> MCASRDDWRCARSMHEFSAKDIDGHMVNLDKYRG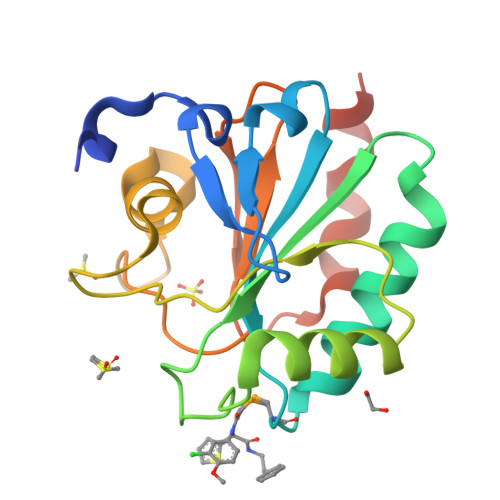FVCIVTNVASQUGKTEVNYTQLVDLHARYAESGLRILAFPCNQFGKQEPGSNEEIKEFAAGYNVKFDMFSKICVNGDDAHPLWKWMKIQPKGKGILGNAIKWNFTKFLIDKNGCVVKRYGPMEEPLVIEKDLPHYFHHHHHH> MMFRGTSCALARSFRANLKYPSLVSYNKLPWEVVSHDSTKLHMHLAPNYEQLLTLAAVTDVPHLTLAS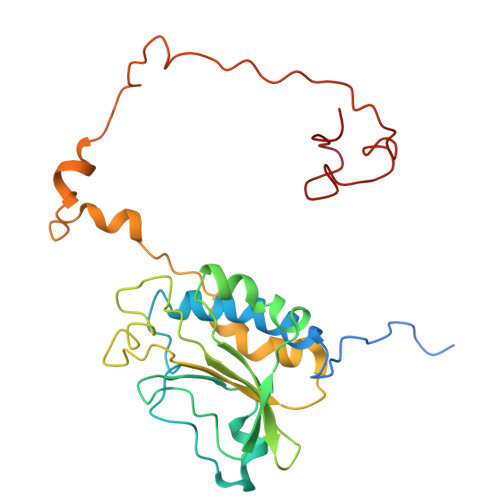HLIVPEAERLRVMPGVVYLLGGQAAHENPSSFTAYRIADPTSLQYYGRIHHNLAPIRRVDMCASADLRLLCLAMHFDGVLTNTSAGSTLDGVTTASQEGHFSLFYFFRPNRPANELTQPFEKFYRHRPSLASLDAFNAASPGKAESWTPVLQVPRRTAEKARLTPAEPYRPPQNYLMGLAERLGVRPGNAFGRRSLMWGTWF> GSGKRGLAYNNINLLTA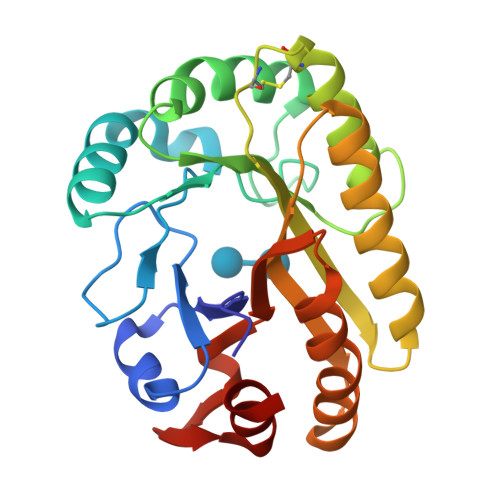FEGGPFSWSYNWEPRPGGYTAGIEYVPMLWGPRGYGSWNADAEAGIAAGSKNLLAFNEPDIASQANMSPEAAAAAYQKYMNPYAARARLGSPAVSNGAPPKGLGWMQGFLDVCAGNCKIDFLAVHWHGPSGNVDDFKRYVSEAIALGQKYGIGTVWVTEFEGQGDEEAQVNFLKEVLPWLDSNAGVERYASFFVDNLVKGGALTSVGKAYKTI>[2x]VACPDGVHTASNAACCAWFPVLDDIQQNLFHGGQCGAEAHEALRMVFHDSIAISPKLQSQGKFGGGGADGSIITFSSIETTYHPNIGLDEVVAIQKPFIAKHGVTPGDFIAFAGAVGVSNCPGAPQMQFFLGRPEATQAAPDGLVP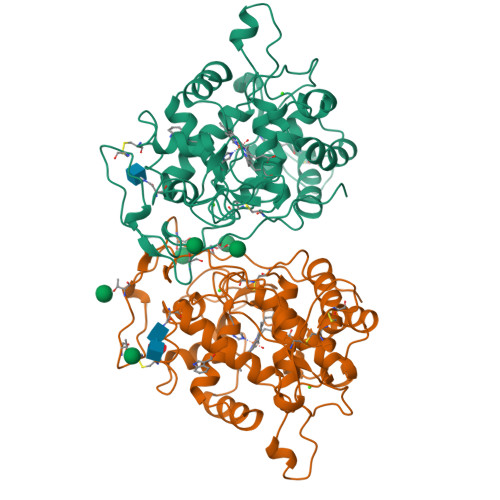EPFHTIDQVLARMLDAGGFDEIETVWLLSAHSIAAANDVDPTISGLPFDSTPGQFDSQFFVETQLRGTAFPGKTGIQGTVMSPLKGEMRLQTDHLFARDSRTACEWQSFVNNQTKLQEDFQFIFTALSTLGHDMNAMIDCSEVIPAPKPVNFGPSFFPAGKTHADIEQACASTPFPTLITAPGPSASVARIPPPPSPNW> MAEASSANLGSGCEEKRHEGSSSESVPPGTTISRVKLLDTMVDTFLQKLVAAGSYQRFTDCYKCFYQLQPAMTQQIYDKFIAQLQTSIREEISDIKEEGNLEAVLNALDKIVEEGKVRKEPAWRPSGIPEKDLHSVMAPYFLQQRDTLRRHVQKQEAENQQLA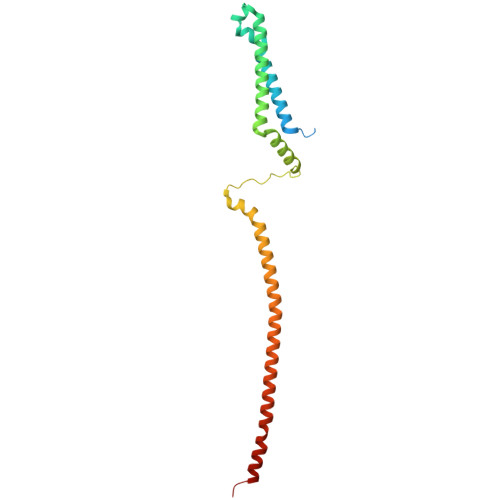DAVLAGRRQVEELQLQVQAQQQAWQALHREQRELVAVLREPE> MKHHHHHHSAGLEVLFQGPGTGSEFELMMFGKKKNNGGSSTARYSAGNKYNTLSNNYALSAQQLLNASKIDDIDSMMGFERYVPPQYNGRFDAKDIDQIPGRVGWLTNMHATLVSQETLSSGSNGGGNSNDGERVTTNQGISGVDFYFLDEEGGSFKSTVVYDPYFFIACNDESRVNDVEELVKKYLESCLKSLQIIRKEDLTMDNHLLGLQKTLIKLSFVNSNQLFEARKLLRPILQDNANNNVQRNIYNVAANGSEKVDAKHLIEDIREYDVPYHVRVSIDKDIRVGKWYKVTQQGFIEDTRKIAFADPVVMAFAIATTKPPLKFPDSAVDQIMMISYMIDGEGFLITNREIISEDIEDFEYTPKPEYPGFFTIFNENDEVALLQRFFEHIRDVRPTVISTFNGDFFDWPFIHNRSKIHGLDMFDEIGFAPDAEGEYKSSYCSHMDCFRWVKRDSYLPQGSQGLKAVTQSKLGYNPIELDPELMTPYAFEKPQHLSEYSVSDAVATYYLYMKYVHPFIFSLCTIIPLNPDETLRKGTGTLCEMLLMVQAYQHNILLPNKHTDPIERFYDGHLLESETYVGGHVESLEAGVFRSDLKNEFKIDPSAIDELLQELPEALKFSVEVENKSSVDKVTNFEEIKNQITQKLLELKENNIRNELPLIYHVDVASMYPNIMTTNRLQPDSIKAERDCASCDFNRPGKTCARKLKWAWRGEFFPSKMDEYNMIKRALQNETFPNKNKFSKKKVLTFDELSYADQVIHIKKRLTEYSRKVYHRVKVSEIVEREAIVCQRENPFYVDTVKSFRDRRYEF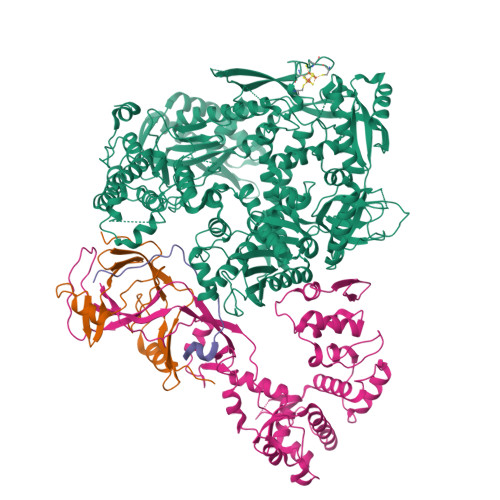KGLAKTWKGNLSKIDPSDKHARDEAKKMIVLYDSLQLAHKVILNSFYGYVMRKGSRWYSMEMAGITCLTGATIIQMARALVERVGRPLELDTDGIWCILPKSFPETYFFTLENGKKLYLSYPCSMLNYRVHQKFTNHQYQELKDPLNYIYETHSENTIFFEVDGPYKAMILPSSKEEGKGIKKRYAVFNEDGSLAELKGFELKRRGELQLIKNFQSDIFKVFLEGDTLEGCYSAVASVCNRWLDVLDSHGLMLEDEDLVSLICENRSMSKTLKEYEGQKSTSITTARRLGDFLGEDMVKDKGLQCKYIISSKPFNAPVTERAIPVAIFSADIPIKRSFLRRWTLDPSLEDLDIRTIIDWGYYRERLGSAIQKIITIPAALQGVSNPVPRVEHPDWLKRKIAT;> MSINLHSAPEYDPSYKLIQLTPELLDIIQDPVQNHQLRFKSLDKDKSEVVLCSHDKTWVLKQRKHSNTVLLMREFVPEQPITFDETLLFGLSKPYMDVVGFAKTESEFETRETHGELNLNSVPIYNGELDFSDKIMKRSSTKVIGTLEELLENSPCSALEGISKWHKIGGSVKDGVLCILSQDFLFKALHVLLMSAMAESLDLQHLNVEDTHHAVGKDIEDEFNPYTREIIETVLNKFAVQEQEAENNTWRLRIPFIAQWYGIQALRKYVSGISMPIDEFLIKWKSLFPPFFPCDIDIDMLRGYHFKPTDKTVQYIAKSTLPMDPKERFKVLFRLQSQWDLEDIKPLIEELNSRGMKIDSFIMKYARRKRLGKKTVVTSR;> MPSVDIDASQWQKLTQSREKQTTVITPLGMMMLEIQGELELPKDFASLARRDSPNEGRFSEQDGETLIRFGSLQIDGERATLFVGKKQRLLGKVTKLDVPMGIMHFNSKDNKVELVDVMKYKVIFKDRPLPIM;> GAMGNQTVKIWVKYNEGFSNAVRKNVTWNNLWE>AAVILESIFLKRSQQKKKTSPLNFKKRLFLLTVHKLSYYEYDFERGRRGSKKGSIDVEKITCVETVVPEKNPPPERQIPR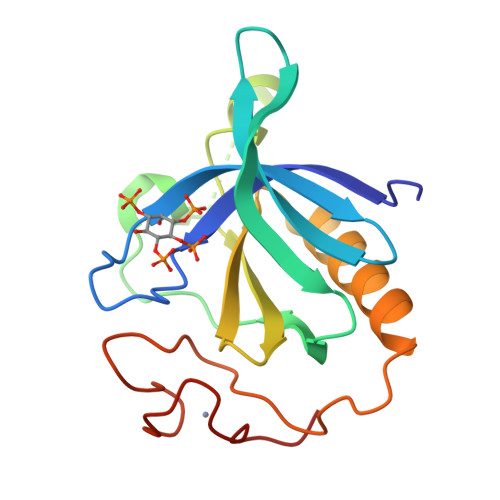RGEESSEMEQISIIERFPYPFQVVYDEGPLYVFSPTEELRKRWIHQLKNVIRYNSDLVQKYHPCFWIDGQYLCCSQTAKNAMGCQILEN[4x]>[2x]MFLKRLDVIGFKSFAERISVDFVKGVTAVVGPNGSGKSNITDAIRWVLGEQSARSLRGGKMEDIIFAGSDSRKRLNLAEVTLTLDNDDHFLPIDFHEVSVTRRVYRSGESEFLINNQPCRLKDIIDLFMDSGLGKEAFSIISQGKVEEILSSKAEDRRSIFEEAAGVLKYKTRKKKAENKLFETQDNLNRVEDILHELEGQVEPLKIQASIAKDYLEKKSGGSLIKLAIEELGTVNLGSIDEFERVNERYKFLSEQKEDLTEAKNTLFQVIEEMDEEMTKRFNDTFVQIRSHFDQVFRSLFGGGRAELRLTDPNDLLHSGVEIIAQPPGKKLQNLNLLSGGERALTAIALLFSILKVRPVPFCVLDQVEAALDEANVFRFAQYLKKYSSDTQFIVITHRKGTMEEADVLYGVTMQESGVSKVISVKLEETKEFVQ;>NRPMETTITRQDIPIEARMNEIVHSLKS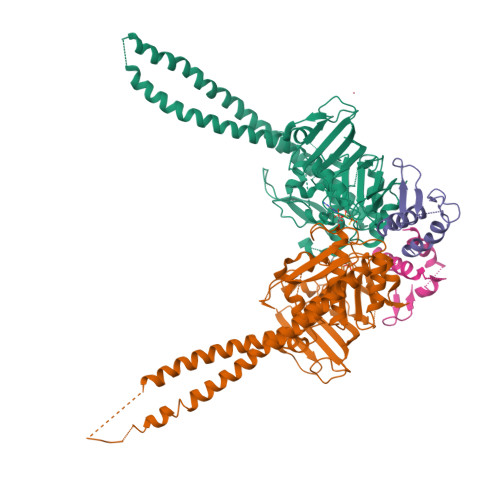RGTRINFMDLFPYEQKEHLVVTFLAVLELMKNQLVLIEQEHNFSDIYITGSESIHGAVDKL[2x]> MAYHKKVVDHYENPRNVGSLDKTSKNVGTGLVGAPACGDVMKLQIQVDEKGKIVDARFKTFGCGSAIASSSLATEWVKGKTVEEALTIKNTDIAKELCLPPVKLHCSMLAEDAIKAALADYKLK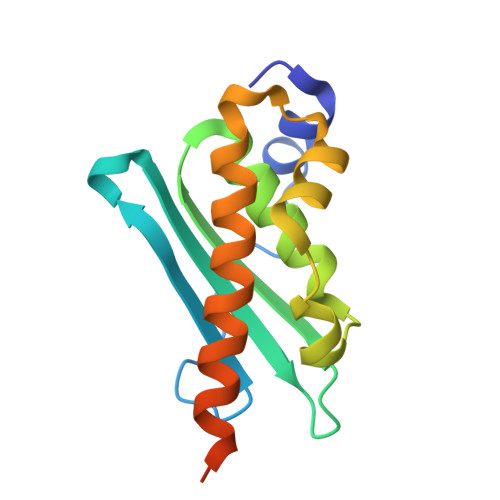QEPKKGEAEKKLEHHHHHH> MKDLLNLLKNQGQIEEFDAIRIGLASPEMIRSWSFGEVKKPETINYRTFKPERDGLFCAKIFGPVKDYECLCGKYKRLKHRGVICEKCGVEVALAKVRRERMGHIELASPVAHIWFLKSLPSRIGLLLDMTLRDIERVLYFESYVVIDPGMTTLEKGQLLNDEQYFEALEEFGDDFDARMGAEAVHELLNAIDLEHEIGRLREEIPQTNSETKIKKLSKRLKLMEAFQGSGNKPEWMVLTVLPVLPPDLRPLVPLDGGRFATSDLNDLYRRVINRNNRLKRLLDLAAPDIIVRNEKRMLQEAVDALLDNGRRGRAITGSNKRPLKSLADMIKGKQGRFRQNLLGKRVDYSGRSVITVGPTLRLHQCGLPKKMALELFKPFIFGKLEGRGMATTIKAAKKMVERELPEVWDVLAEVIREHPVLLNRAPTLHRLGIQAFEPVLIEGKAIQLHPLVCAAYNADFDGDQMAVHVPLTLEAQLEARALMMSTNNILSPANGEPIIVPSQDVVMGLYYMTREAINAKGEGMAFADLQEVDRAYRSGQASLHARVKVRINEKIKGEDGQLTANTRIVDTTVGRALLFQVVPAGLPFDVVNQSMKKKAISKLINHCYRVVGLKDTVIFADQLMYTGFAYSTISGVSIGVNDFVIPDEKARIINAATDEVKEIESQYASGLVTQGEKYNKVIDLWSKANDEVSKAMMANLSKEKVVDREGKEVDQESFNSMYMMADSGARGSAAQIRQLAGMRGLMAKPDGSIIETPITANFREGLNVLQYFISTHGARKGLADTALKTANSGYLTRRLVDVAQDLVVTEIDCGTEHGLLMSPHIEGGDVVEPLGERVLGRVIARDVFKPGSDEVIVPAGTLIDEKWVDFLEVMSVDEVVVRSPITCETRHGICAMCYGRDLARGHRVNIGEAVGVIAAQSIGEPGTQLTMRTFHIGGAASRTSAADNVQVKNGGTIRLHNLKHVVRADGALVAVSRSGELAVADDFGRERERYKLPYGAVISVKEGDKVDPGAIVAKWDPHTHPIVTEVDGTVAFVGMEEGITVKRQTDELT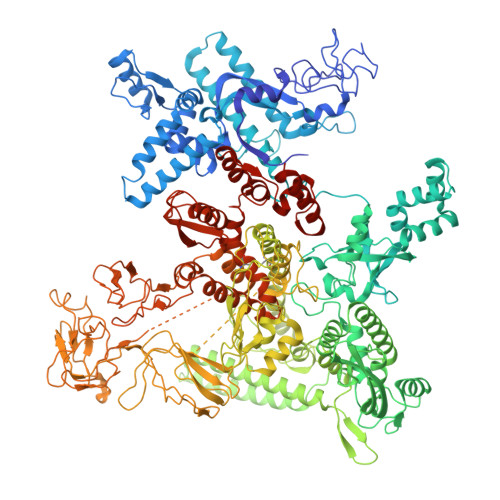GLTNIEVMDPKDRPAAGKDIRPAVKLIDAAGKDLLLPGTDVPAQYFLPANALVNLTDGAKVSIGDVVARIPQETSKTRDITGGLPRVADLFEARRPKEPSILAEISGTISFGKETKGKRRLVITPNDGSDPYEELIPKWRHLNVFEGEQVNRGEVISDGPSNPHDILRLLGVSSLAKYIVNEIQDVYRLQGVKINDKHIETILRQMLRKVEVSESGDSSFIKGDQVELTQVLEENEQLGTEDKFPAKYERVLLGITKASLSTESFISAASFQETTRVLTEAAVTGKRDFLRGLKENVVVGRLIPAGTGLAYHSERKRQRDLGKPQRVSASEAEAALTEALNSSGN>[2x]MKYQQLENLESGWKWAYLVKKHRE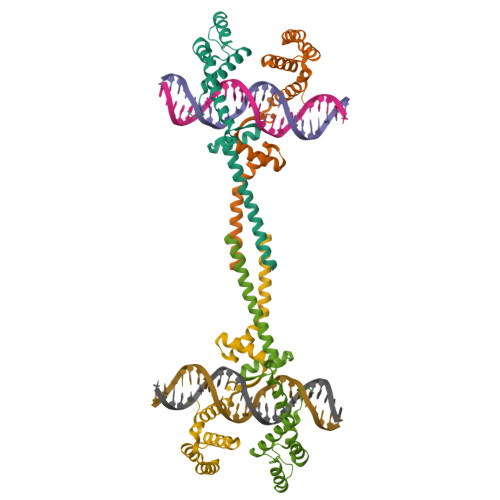GEAITRHIENSAAQDAVEQLMKLENEPVKVQEWIDAHMNVNLATRMKQTIRARRKRHFNAEHQHTRKKSIDLEFLVWQRLAVLARRRGNTLSDTVVQLIEDAERKEKYASQMSSLKQDLKDILDKEV>AMDPMKIADLMTLLDHHVPFSTAESWDNVGLLIGDEDVEVTGVLTALDCTLEVVNEAIEKGYNTIISHHPLIFKGVTSLKANGYGLIIRKLIQHDINLIAMHTNLDVNPYGVNMMLAKVMGLKNISIINNQQDVYYKVQTYIPKDNVGPFKDKLSENGLAQEGNYEYCFFESEGRGQFKPVGEANPTIGQIDKIED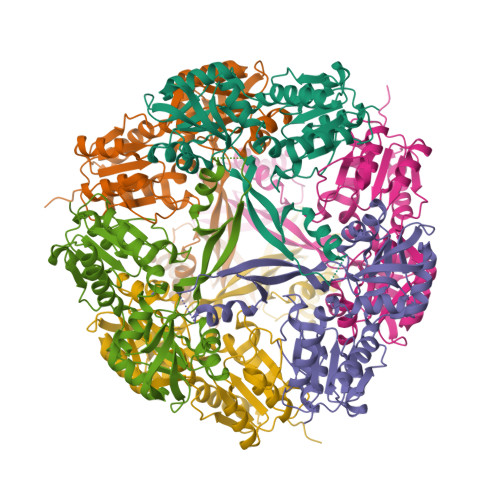VDEVKIEFMIDAYQKSRAEQLIKQYHPYETPVFDFIEIKQTSLYGLGVMAEVDNQMTLEDFAADIKSKLNIPSVRFVGESNQKIKRIAIIGGSGIGYEYQAVQQGADVFVTGDIKHHDALDAKIHGVNLIDINHYSEYVMKEGLKTLLMNWFNIEKINIDVEASTINTDPFQYI[2x]>MKEFYISIETVGNNIVERYIDENGKERTREVEYLPTMFRHCKEESKYKDIYGKNCAPQKFPSMKDARDWMKRMEDIGLEALGMNDFKLAYISDTYGSEIVYDRKFVRVANCDIEVTGDKFPDPMKAEYEIDAITHYDSIDDRFYVFDLLNSMYGSVSKWDAKLAAKLDCEGGDEVPQEILDRVIYMPFDNERDMLMEYINLWEQKRPAIFTGWNIEGFAVPYIMNRVKMILGERSMKRFSPIGRVKSKLIQNMYGSKEIYSIDGVSILDYLDLYKKFAFTNLPSFSLESVAQHETKKGKLPYDGPINKLRETNHQRYISYNIIDVESVQAIDKIRGFIDLVLSMSYYAKMPFSGVMSPIKTWDAIIFNSLKGEHKVIPQQGSHVKQSFPGAFVFEPKPIARRYIMSFDLTSLYPSIIRQVNISPETIRGQFKVHPIHEYIAGTAPKPSDEYSCSPNGWMYDKHQEGIIPKEIAKVFFQRKDWKKKMFAEEMNAEAIKKIIMKGAGSCSTKPEVERYVKFSDDFLNELSNYTESVLNSLIEECEKAATLANTNQLNRKILINSLYGALGNIHFRYYDLRNATAITIFGQVGIQWIARKINEYLNKVCGTNDEDFIAAGDTDSVYVCVDKVIEKVGLDRFKEQNDLVEFMNQFGKKKMEPMIDVAYRELCDYMNNREHLMHMDREAISCPPLGSKGVGGFWKAKKRYALNVYDMEDKRFAEPHLKIMGMETQQSSTPKAVQEALEESIRRILQEGEESVQEYYKNFEKEYRQLDYKVIAEVKTANDIAKYDDKGWPGFKCPFHIRGVLTYRRAVSGLGVAPILDGNKVMVLPLREGNPFGDKCIAWPSGTELPKEIRSDVLSWIDHSTLFQKSFVKPLAGMCESAGMDYEEKASLDFLFG[2x];>MKLSKDTTALLKNFATINSGIMLKSGQFIMTRAVNGTTYAEANISDVIDFDVAIYDLNGFLGILSLVNDDAEISQSEDGNIKIADARSTIFWPAADPSTVVAPNKPIPFPVASAVTEIKAEDLQQLLRVSRGLQIDTIAITVKEGKIVINGFNKVEDSALTRVKYSLTLGDYDGENTFNFIINMANMKMQPGNYKLLLWAKGKQGAAKFEGEHANYVVALEADSTHDF[3x]

The T4 replication system centers on a holoenzyme complex that is assembled from the DNA polymerase (gp43) and the sliding clamp (gp45) loaded onto a primer/template junction by the clamp loader complex (gp44/62) in the presence of ATP. The sliding clamp plays a crucial role by encircling the DNA double helix and anchoring the polymerase to the template. Sequence analysis reveals that T4 polymerase contains three main structural regions: an N-terminal domain, a 3′-5′ exonuclease domain responsible for proofreading activity, and a C-terminal polymerase domain. The T4 gp45 sliding clamp forms a trimeric ring structure, with each of the three monomers composed of structurally similar N-terminal and C-terminal domains (NTD and CTD).

In state 2, both thumb domains align at equivalent heights. DNA interaction is restricted to the left polymerase, where thumb residues Arg-704, Phe-796, Lys-797, and Arg-803 engage the substrate, while the right polymerase maintains no DNA contacts. The primer 3′-end occupies neither catalytic site of the left polymerase. In state 2, the DNA occupies the central region of the clamp channel, maintaining proximity to all three Arg-131 residues from each clamp monomer. In both states 1 and 2, the DNA substrate remains displaced from the polymerization active site in either polymerase, with the primer 3′ terminus positioned 16 Å away from the catalytic residue Asp-620 and the finger domain maintaining an open conformation. During the transition from state 3 to state 2, the duplex region of the DNA moves toward the clamp’s central channel and becomes less severely tilted. This shift causes the primer/template DNA to disengage from the left polymerase and move 14 Å toward the right polymerase. Superposition of the right polymerases of states 2 and 3 illuminates the structural rearrangements required to reposition the DNA primer from its inactive placement in the left polymerase of state 2 to the catalytically competent configuration observed in state 3. This alignment reveals four coordinated transitions: (i) further upward tilting of the sliding clamp relative to the DNA; (ii) downward compression of the polymerase thumb for improved DNA engagement; consequently, (iii) P/T DNA rotation that shifts the template strand laterally by 16 Å to optimize interactions with the thumb; and (iv) finger domain closure to stabilize the incoming nucleotide.>HHHHHHMTVVDAVSTDAAGAAPAAAAAPVVVAQPGNGQTVCVTGAAGYIASWLVKMLLEKGYTVKGTVRNPDDPKNAHLKALDGAAERLILCKADLLDYDAICRAVQGCQGVFHTASPVTDDPEQMVEPAVRGTEYVINAAAEAGTVRRVVFTSSIGAVTMDPSRGPDVVVDESCWSDLEFCKKTRNWYCYGKAVAEQAAWDAARQRGVDLVVVNPVLVVGPLLQPTVNASIAHVLKYLDGSARTFANAVQAYVDVRDVADAHLRVFESPAASGRYLCAERVLHREDVVRILAKLFPEYPVPTRCSDEVNPRKQPYKFSNQKLRD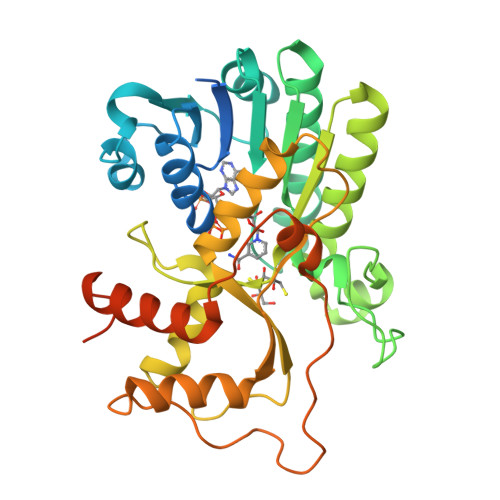LGLEFRPVSQSLYDTVKNLQEKGHLPVLGEQTTEADKEEANAAAEVQQGGIAIRA[2x]>[6x]GSHGMGQATAIAHPNIAFIKYWGKRDAVLRIPENGSISMNLAELTVKTTVIFEKHSREDTLILNGALA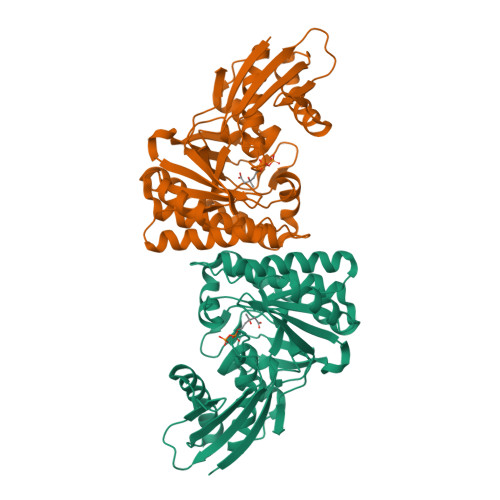DEPALKRVSHFLDRVREFAGISWHAHVISENNFPTGAGIASSAAAFAALALAATSAIGLHLSERDLSRLARKGSGSACRSIPGGFVEWIPGETDEDSYAVSIAPPEHWALTDCIAILSTQHKPIGSTQGMALASTSPLQPARVADTPRRLEIVRRAILERDFLSLAEMIEHDSNLMHAVMMTSTPPLFYWEPVSLVIMKSVREWRESGLPCAYTLDAGPNVHVICPSEYAEEVIFRLTSIPGVQTVLKASAGDSAKLIEQSL>[2x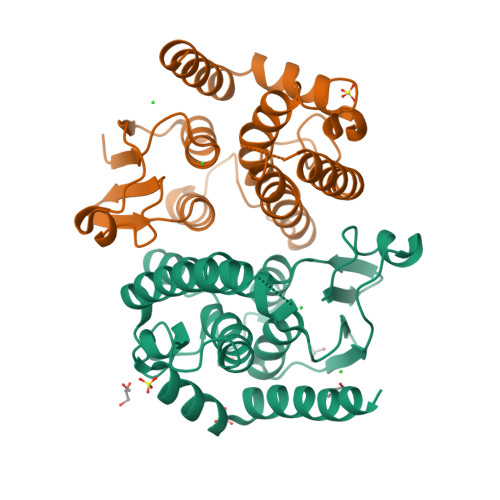]MVMIKLHGASISNYVNKVKLGILEKGLEYEQIRIAPSQEEDFLKISPMGKIPVLEMDGKFIFESGAILEFLDTIFPQTPKLIPEDPWEAARVREISTIIETYLDIPARRIYLPAAKVSPEIVEEVHSTLVKGIKALQRVVRFSPYIAGNVFTLADCSGFAHLSVLDEELRPFYPNNHPLDLLNGWKEYFVFMKTKAGPALVEKDKQILKKILARAKTKIGAENLYFQSHHHHHHWSHPQFEK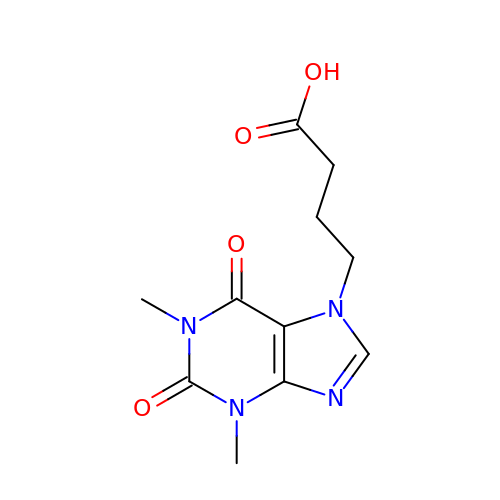4-(1,3-dimethyl-2,6-dioxo-1,2,3,6-tetrahydro-7H-purin-7-yl)butanoic acid | C11 H14 N4 O4 | KCQMWMWEALWVLJ-UHFFFAOYSA-N> GSSHHHHHHSSGLVPRGSMSTSWSDRLQNAA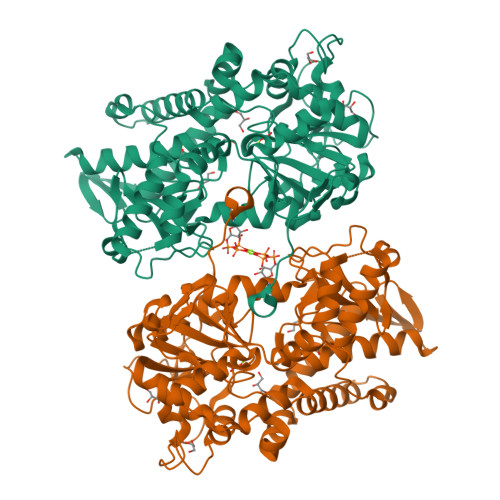DMPANMDKHALKKYRREAYHRVFVNRSLAMEKIKCFGFNMDYTLAVYKSPEYESLGFELTVERLVSIGYPQELLSFAYDSTFPTRGLVFDTLYGNLLKVDAYGNLLVCAHGFNFIRGPETREQYPNKFIQRDDTERFYILNTLFNLPETYLLACLVDFFTNCPRYTSCETGFKDGDLFMSYRSMFQDVRDAVDWVHYKGSLKEKTVENLEKYVVKDGKLPLLLSRMKEVGKVFLATNSDYKYTDKIMTYLFDFPHGPKPGSSHRPWQSYFDLILVDARKPLFFGEGTVLRQVDTKTGKLKIGTYTGPLQHGIVYSGGSSDTICDLLGAKGKDILYIGDHIFGDILKSKKRQGWRTFLVIPELAQELHVWTDKSSLFEELQSLDIFLAELYKHLDSSSNERPDISSIQRRIKKVTHDMDMCYGMMGSLFRSGSRQTLFASQVMRYADLYAASFINLLYYPFSYLFRAAHVLMPHESTVEHTHVDINEMESPLATRNRTSVDFKDTDYKRHQLTRSISEIKPPNL> MHQPKKRLAKKSWAFLTAALTLGVITGVGGYFLFNQNKQRSSVSNFAYQPKQLSVKHQQAVDETLTPWTWNNNNFSSLKITGENPGSFGLVRSQNDNLNISSVTKNSSDDNLKYLNAVEKYLDGQQNFAIRRYDNNGRALYDINLAKMENPSTVQRGLNGEPIFDPFKGFGLTGNAPTDWNEIKGKVPVEVVQSPHSPNLYFVLLVPKVALEYHNLNNQVVKESLEVKATQSSFNPTQRLQKDSPV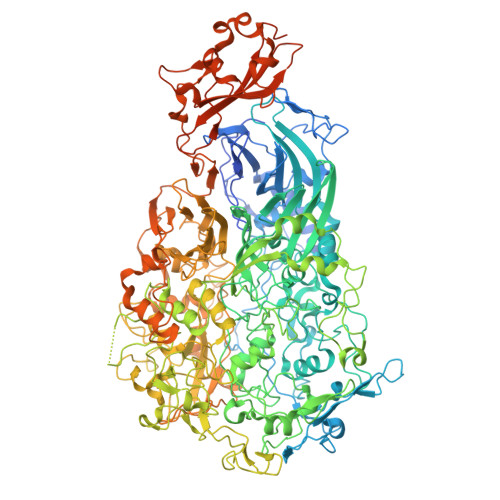KDSSKQGEKLSETTASSMSSGMATSTRAKALKVEVERGSQSDSLLKNDFAKKPLKHKNSSGEVKLEAEKEFTEAWKPLLTTDQIAREKGMGATVVSFYDAPYSENHTAFGLVDHIDPKKMVENYPPSWKTPKWNHHGIWDYNARNLLLQTTGFFNPRRHPEWFDEGQAKADNTSPGFKVGDTDHKKDGFKKNSSSPIALPFEAYFANIGNMVAIGNSVFIFGGNGHATKMFTTNPLSIGVFRIKYTDNFSKSSVTGWPYAVLFGGLINPQTNGLKDLPLGTNRWFEYVPRMAVSGVKWVGNQLVLAGTLTMGDTATVPRLKYDQLEKHLNLVAQGQGLLREDLQIFTPYGWANRPDIPVGAWLQDEMGSKFGPHYFLNNPDIQDNVNNDTVEALISSYKNTDKLKHVYPYRYSGLYAWQLFNWSNKLTNTPLSANFVNENSYAPNSLFAAILNEDLLTGLSDKIFYGKENEFAENEADRFNQLLSLNPNPNTNWARYLNVVQRFTTGPNLDSSTFDQFLDFLPWIGNGKPFSNSPSPSTSASSSTPLPTFSNINVGVKSMITQHLNKENTRWVFIPNFSPDIWTGAGYRVQSANQKNGIPFEQVKPSNNSTPFDPNSDDNKVTPSGGSSKPTTYPALPNSISPTSDWINALTFTNKNNPQRNQLLLRSLLGTIPVLINKSGDSNDQFNKDSEQKWDKTETNEGNLPGFGEVNGLYNAALLHTYGFFGTNTNSTDPKIGFKADSSSSSSSTLVGSGLNWTSQDVGNLVVINDTSFGFQLGGWFITFTDFIRPRTGYLGITLSSLQDQTIIWADQPWTSFKGSYLDSDGTPKSLWDPTALKSLPNSSTTYDTNPTLSPSFQLYQPNKVKAYQTTNTYNKLIEPVDATSAATNMTSLLKLLTTKNIKAKLGKGTASSQGNNNGGGVSQTINTITTTGNISEGLKEETSIQAETLKKFFDSKQNNKSEIGIGDSTFTKMDGKLTGVVSTPLVNLINGQGATSDSDTEKISFKPGNQIDFNRLFTLPVTELFDPNTMFVYDQYVPLLVNLPSGFDQASIRLKVISYSVENQTLGVRLEFKDPQTQQFIPVLNASSTGPQTVFQPFNQWADYVLPLIVTVPIVVIILSVTLGLTIGIPMHRNKKALQAGFDLSNKKVDVLTKAVGSVFKEIINRTGISNAPKKLKQATPTKPTPKTPPKPPVKQ> MAAAAAGAGSGPWAAQEKQFPPALLSFFIYNPRFGPREGQEENKILFYHPNEVEKNEKIRNVGLCEAIVQFTRTFSPSKPAKSLHTQKNRQFFNEPEENFWMVMVVRNPIIEKQSKDGKPVIEYQEEELLDKVYSSVLRQCYSMYKLFNGTFLKAMEDGGVKLLKERLEKFFHRYLQTLHLQSCDLLDIFGGISFFPLDKMTYLKIQSFINRMEESLNIVKYTAFLYNDQLIWSGLEQDDMRILYKYLTTSLFPRHIEPELAGRDSPIRAEMPGNLQHYGRFLTGPLNLNDPDAKCRFPKIFVNTDDTYEELHLIVYKAMSAAVCFMIDASVHPTLDFCRRLDSIVGPQLTVLASDICEQFNINKRMSGSEKEPQFKFIYFNHMNLAEKSTVHMRKTPSVSLTSVHPDLMKILGDINSDFTRVDEDEEIIVKAMSDYWVVGKKSDRRELYVILNQKNANLIEVNEEVKKLCATQFNNIFFLD;> MATDMQRKRSSECLDGTLTPSDGQSMERAESPTPGMAQGMEPGAGQEGAMFVHARSYEDLTESEDGAASGDSHKEGTRGPPPLPTDMRQISQDFSELSTQLTGVARDLQEEMLPGSSEDWLEPPGAVGRPATEPPREGTTEGDEEDATEAWRLHQKHVFVLSEAGKPVYSRYGSEEALSSTMGVMVALVSFLEADKNAIRSIHADGYKVVFVRRSPLVLVAVARTRQSAQELAQELLYIYYQILSLLTGAQLSHIFQQKQNYDLRRLLSGSERITDNLLQLMARDPSFLMGAARCLPLA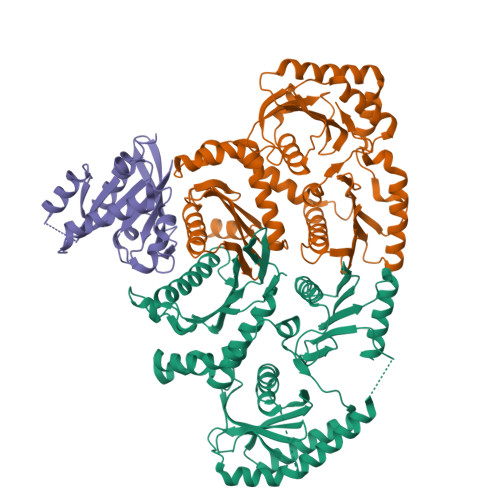AAVRDTVSASLQQARARSLVFSILLARNQLVALVRRKDQFLHPIDLHLLFNLISSSSSFREGEAWTPVCLPKFNAAGFFHAHISYLEPDTDLCLLLVSTDREDFFAVSDCRRRFQERLRKRGAHLALREALRTPYYSVAQVGIPDLRHFLYKSKSSGLFTSPEIEAPYTSEEEQERLLGLYQYLHSRAHNASRPLKTIYYTGPNENLLAWVTGAFELYMCYSPLGTKASAVSAIHKLMRWIRKEEDRLFILTPLTY;> MTSRKKVLLKVIILGDSGVGKTSLMNQYVNKKFSNQYKATIGADFLTKEVMVDDRLVTMQIWDTAGQERFQSLGVAFYRGADCCVLVFDVTAPNTFKTLDSWRDEFLIQASPRDPENFPFVVLGIKIDLENRQVATKRAQAWCYSKNNIPYFETSAKEAINVEQAFQTIARNALKQETEVELYNEFPEPIKLDKNDRAKASAESCSC3-{[(4-bromophenyl)carbamoyl]amino}benzoic acid | C14 H11 Br N2 O3 | 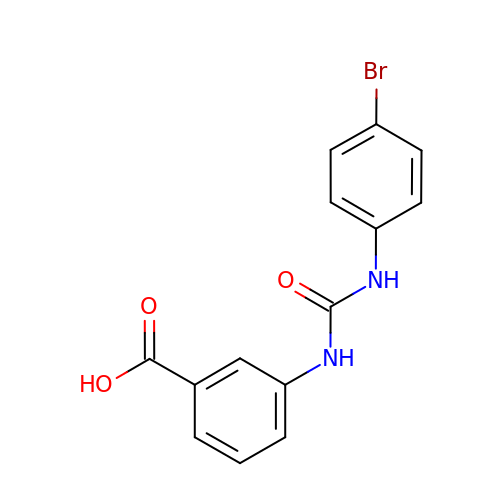XLDDBXYVKMODRJ-UHFFFAOYSA-N The M protein is an essential virulence factor of *Streptococcus pyogenes*, or group A streptococcus (GAS), one of the most common and dangerous human pathogens. Encoded by the chromosomal *emm* gene, the M protein is covalently anchored at its C-terminus to the cell wall, covering the GAS surface at high density and acting as an adhesin and a potent immune evasion factor. The M3 protein is produced by the prevalent *emm*3 GAS serotype, which is frequently associated with severe invasive diseases. To gain insights into mechanism and biological role of streptococcal collagen binding, we characterised the interaction of M3 with the Collagen Ligand Collections (CLCs, triple-helical collagen peptide libraries formerly known as Toolkits), and determined crystal structures of the M3 N-terminal domain (M3-NTD), encompassing the HVR, alone and in complex with a CLC-derived collagen peptide.

M3-NTD includes the 110 N-terminal residues of mature M3 (residues 42-151 of the M3 protein precursor sequence). To stabilize a dimeric conformation, Leu151 was replaced with a cysteine for disulfide bond formation at the C-terminus. M3-NTD crystallized in several conditions with the best crystals diffracting X-rays to a resolution of 1.9 Å at the synchrotron radiation source. M3-NTD is a symmetrical homodimer, linked at the C-terminus by a disulfide bond ([Fig fig5]). The fold represents a novel T-shaped architecture with no significantly similar structures identifiable by the protein structure comparison server DALI. Each monomer is composed of three α-helices, H1-H3. The H3 helices comprise the C-terminal 38 residues of M3-NTD (M3 residues 114-151) and form a coiled coil stem. Helices H1 and H2 form hairpins that pack against each other to form the slightly kinked bar of the T-shape, effectively a three-helix bundle. A key residue is Gly113, which resides at the T-junction, separating H2 and H3 ([Fig fig5]). The T-bar structure is stabilized by a network of polar interactions of several conserved residues, most notably inter-chain salt bridges of Arg52 with Asp102 and Glu105, and an inter-chain hydrogen bond between the side chains of Glu49 and Asn101 ([Fig fig5]).

>[2x]GAMDARSVNGEFPRHVKLKNEIENLLDQVTQLYTKHNSNYQQYNAQAGRLDLRQKAEYLKGLNDWAERLLQELNGEDVKKVLGKVAFEKDDLEKEVKELKEKIDKKEKEYQDC> FSRVVTNADSKAAYVGGADLQALKKFVSEGNKRLDAVNAIVSNASCIVSDAVSGMICENPALISPSGNCYTNRRMAACLRDAEIILRYVSYSLLSGDSSVLEDRCLSGLKETYSSLGVPTAGNLRAVGIMKATCVA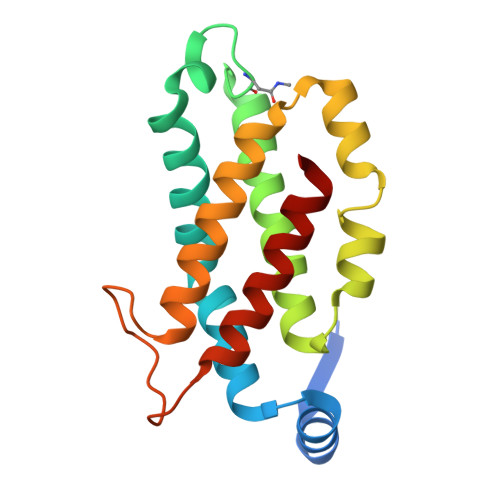FINNTSQQKKLSTPAGDCSALASEVAGYFDKVSAALA> RELHPVAPLLDNLTSAL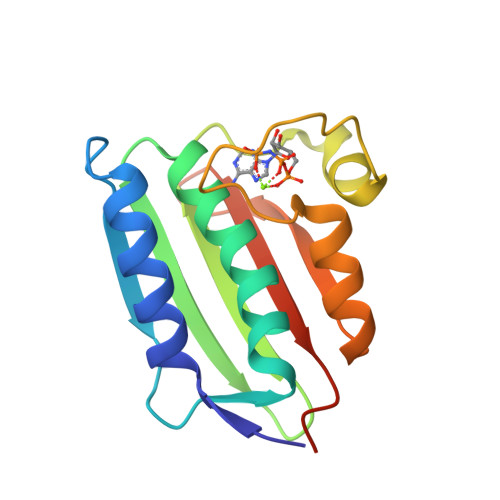NKVYQRKGVNISLDISPEISFVGEQNDFVEVMGNVLDNACKYCLEFVEISARQTDEHLYIVVEDDGPGIPLSKREVIFDRGQRVDTLRPGQGVGLAVAREITEQYEGKIVAGESMLGGARMEVIFGRQHSAPKDE>[2x]MGSSHHHHHHSQDPLEVLFQGPEFMSAIKPDMKIKLRMEGNVNGHHFVIDGDGTGKPFEGKQSMDLEVKEGGPLPFAFDILTTAFHYGNRVFAKYPDNIQDYFKQSFPKG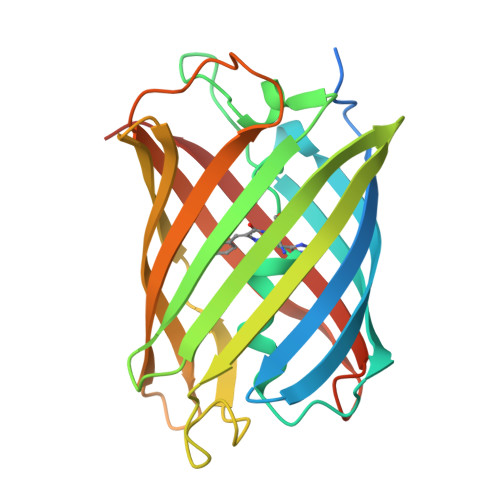YSWERSLTFEDGGICNARNDITMEGDTFYNKVRFYGTNFPANGPVMQKKTLKWEPSTEKMYVRDGVLTGDIEMALLLEGNAHYRCDFRTTYKAKEKGVKLPGAHFVDHCIEILSHDKDYNKVKLYEHAVAHSGLPDNARR>SMEVARAARLAQIFKEICDGIISYKDSSRQALAAPLLNLPPKKKNADYYEKISDPLDLITIEKQILTGYYKTVEAFDADMLKVFRNAEKYYGRKSPVGRDVCRLRKAYYNARHEASAQIDEIVGET[2x]

Bromodomains (BRDs) are protein interaction modules that specifically recognize ε-N-lysine acetylation motifs, a key event in the reading process of epigenetic marks. The 61 BRDs in the human genome cluster into eight families based on structure/sequence similarity. Despite large sequence variations, all BRD modules share a conserved fold that comprises a left-handed bundle of four α helices (αZ, αA, αB, αC), linked by loop regions of variable length (ZA and BC loops), which line the Kac binding site and determine binding specificity. The four helices form a deep cavity that is extended by the two loop regions (ZA and BC loops), creating a largely hydrophobic Kac binding pocket.

BRDs are evolutionarily conserved and present in diverse nuclear proteins comprising HATs (GCN5, PCAF), ATP-dependent chromatin-remodeling complexes (BAZ1B), helicases (SMARCA), methyltransferases (MLL, ASH1L), transcriptional coactivators (TRIM/TIF1, TAFs) transcriptional mediators (TAF1), nuclear-scaffolding proteins (PB1), and the BET family (Muller et al., 2011).> QPIFLNVLEAIEPGVVCAGHDNNQPDSFAALLSSLNELGERQLVHVVKWAKALPGFRNLHVDDQMAVIQYSWMGLMVFAMGWRSFTNVNSAMLYFAPDLVFNEYRMHKSRMYSQCVRMRHLSQEFGWLQITPQEFLCMKALLLFSIIPVDGLKNQKFFDELRMNYIKELDRIIACKRKNP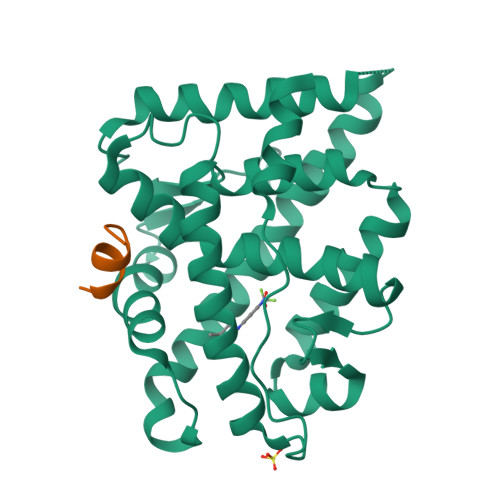TSCSRRFYQLTKLLDSVQPIARELHQFAFDLLIKSHMVSVDFPEMMAEIISVQVPKILSGKVKPIYFHTQ;> KTRYIFDLFYKRKAY> MNASTITLHVPQ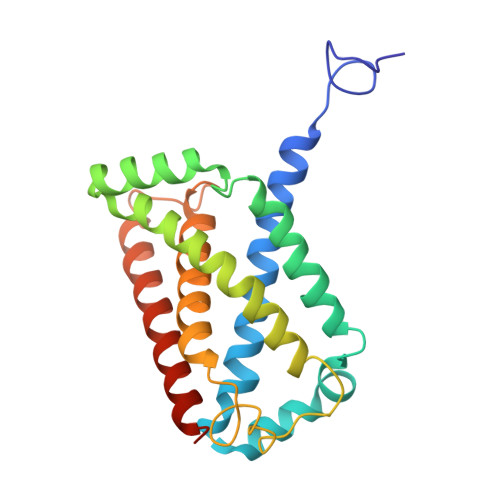RSKIAGRMDFFQMVSGALLILFLWAHMMLVSSVILSPSLMNGIAWFFEATYMAQIGGPAVFVLMVVHFILAARKMPFKQDEWKTFRVHACMLHHKDTTMWVVQVISAIFILVLGAVHMFVVLTDLPITAAKSAARLQSGWLYLYLVLLPLAELHVGVGFYRIGVKYGFVGRNKRKWFQKTENLMMIGFITIGLLTLVRFMLLNIQG> SLGAYLSEPLTTKDSSDESNEFLASGSSSMQGWRISQEDAHNCILNFDDQCSFFAVYDGHGGAEVAQYCSLHLPTFLKTVEAYGRKEFEKALKEAFLGFDATLLQEKVIEELKVLSGDSAGSDAEPGKDSGCTAVVALLHGKDLYVANAGDSRCVVCRNGKALEMSF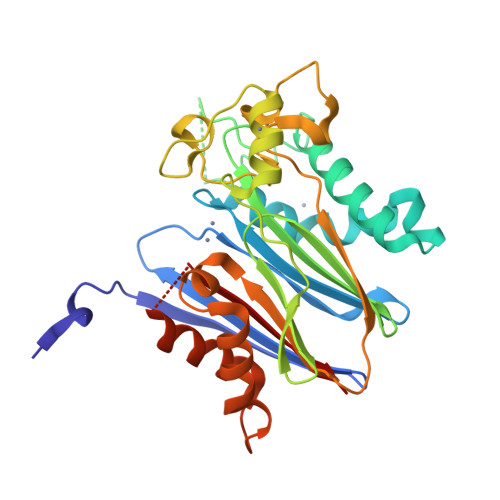DHKPEDTVEYQRIEKAGGRVTLDGRVNGGLNLSRAIGDHGYKMNKSLPAEEQMISALPDIEKITVGPEDEFMVLACDGIWNFMTSEQVVQFVQERINKPGMKLSKICEELFDHCLAPHTRGDGTGCDNMTAIIVQFK> VIVTRSGAILPKPVKMSFGLLR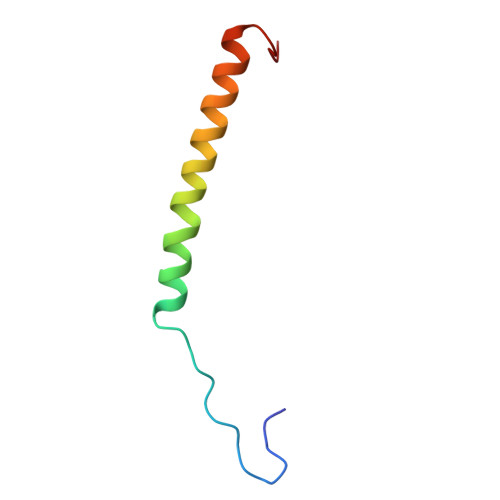VFSIVIPFLYVGTLISKNFAALLEEHDIFVPE> MTATVLLEVPFSARGDRIPDAVAELRTREPIRKVRTITGAEAWLVSSYALCTQVLEDRRFSMKETAAAGAPRLNALTVPPEVVNNMGNIADAGLRKAVMKAITPKAPGLEQFLRDTANSLLDNLITEGAPADLRNDFADPLATALHCKVLGIPQEDGPKLFRSLSIAFMSSADPIPAAKINWDRDIEYMAG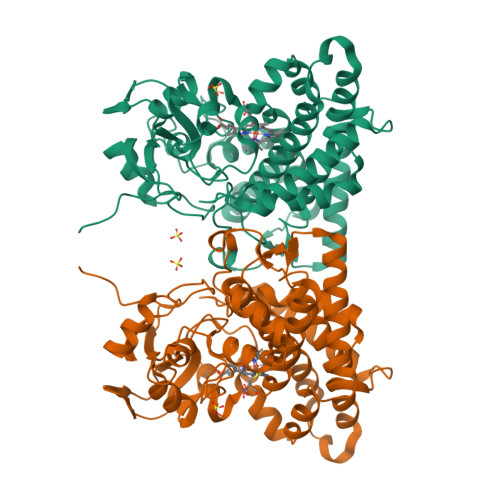ILENPNITTGLMGELSRLRKDPAYSHVSDELFATIGVTFFGAGVISTGSFLTTALISLIQRPQLRNLLHEKPELIPAGVEELLRINLSFADGLPRLATADIQVGDVLVRKGELVLVLLEGANFDPEHFPNPGSIELDRPNPTSHLAHGRGQHFCPGSALGRRHAQIGIEALLKKMPGVDLAVPIDQLVWRTRFQRRIPERLPVLW> GHMNPEYDYLFKLLLIGDSGVGKSCLLLRFADDTYTESYISTIGVDFKIRTIELDGKTIKLQIWDTAGQERFRTITSSYYRGAHGIIVVYDVTDQESYANVKQWLQEIDR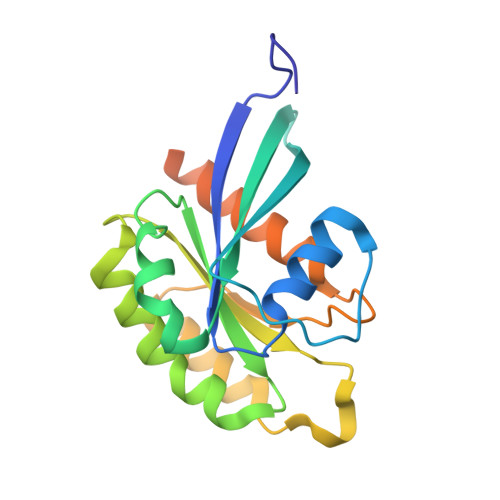YASENVNKLLVGNKSDLTTKKVVDNTTAKEFADSLGIPFLETSAKNATNVEQAFMTMAAEIKKRMGPGAASGGERPNLKIDSTPVKPAGGGCC1-(4-{3,5-dichloro-4-[(2,6-dimethylpyridin-3-yl)methoxy]phenyl}pyridin-2-yl)piperazine 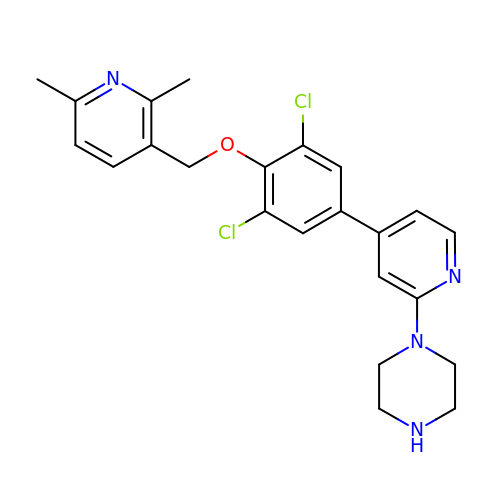| C23 H24 Cl2 N4 O | RMXRTRBIKXITFB-UHFFFAOYSA-N> SIQAEEWYFGKITRRESERLLLNAENPRGTFLVRESETTKGAYCLSVSD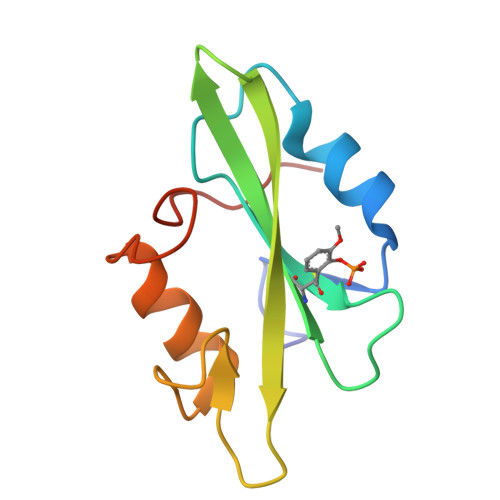FDNAKGLNVKHYKIRKLDSGGFYITSRTQFNSLQQLVAYYSKHADGLCHRLTTVCPTSK>GAMASSSHSRAGQSAAGAAPGGGVDTRDAEMPATEKDLAEDAPWKKIQQNTFTRWCNEHLKCVSKRIANLQTDLSDGLRLIALLEVLSQKKMHRKHNQRPTFRQMQLENVSVALEFLDRESIKLVSIDSKAIVDGNLKLILGLIWTLILHYSISMPMWDEEEDEE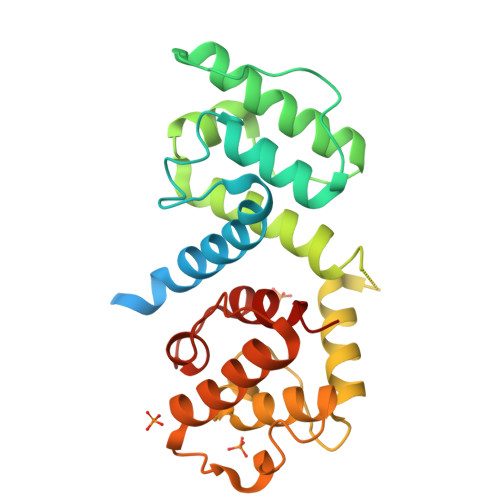AKKQTPKQRLLGWIQNKLPQLPITNFSRDWQSGRALGALVDSCAPGLCPDWDSWDASKPVTNAREAMQQADDWLGIPQVITPEEIVDPNVDKHSVMTYLSQFPKAKL[2x]>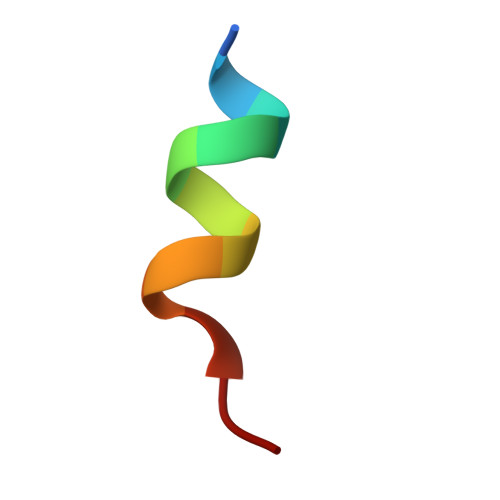 AARDAAVSDAAA> MQDNSRYTHFLTQHYDAKPQGRDDRYCESIMRRRGLTSPCKDINTFIHGNKRSIRAICENKNGNPHRENLRISKSSFQVTTCKLHG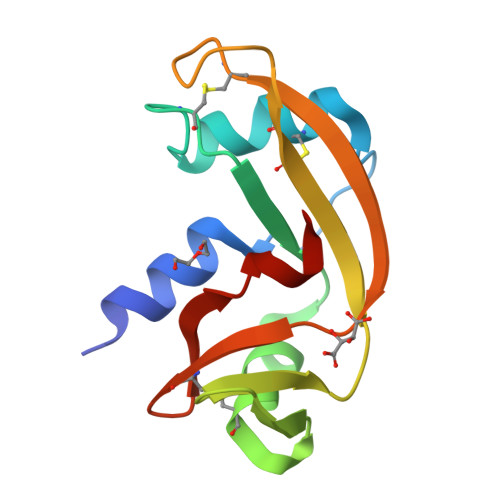GSPWPPCQYRATAGFRNVVVACENGLPVHLDQSIFRRP ChdCs are enzymes involved in the prokaryotic heme biosynthesis pathway mainly of monoderm bacteria, but some diderm or intermediate representatives also use this pathway. They catalyze the hydrogen peroxide–driven oxidative decarboxylation of iron coproporphyrin III (coproheme) to iron protoporphyrin IX (heme b). After initial oxidation of coproheme to Compound I (two-electron deficient reaction intermediate), a catalytic tyrosine radical is generated, which is completely essential for both decarboxylation reactions. Mechanistic studies revealed the order of decarboxylation and proved that propionate at position 2 (p2) is decarboxylated first.

Exchange of Y135 with a tryptophan, in order to mirror the situation in the active site, led to a very inactive variant (data not shown), we therefore eliminated Y135 by inserting an alanine residue (Y135A), as has proven to keep the formation of Compound I perfectly intact in previous studies. The structures clearly show that the introduced amino acids occupy the positions of the respective residues in the wild-type protein. While the distance between Y135 and Cß-p2 is about 3.1 Å in the wild-type structure, the Y183 oxygen lies about 4.4 Å above the Cß of p4. Both single mutations leave the active site and the overall structure is unaffected. Y135A, in contrast, exhibits a very similar UV–Vis spectrum to the wild type (Soret maximum at 391 with a shoulder, visible bands at 490 and 631 nm) but shows no spectral shift of the Soret maximum upon titration with H2O2. Instead, an absorbance decrease of the Soret maximum and emergence of a single band at 580 nm are observed. As there is a lack of catalytic Y135, no decarboxylation activity with H2O2 is observed in this variant. Y135A is unable to perform the decarboxylation reaction on coproheme. This variant will form Compound I in the presence of H2O2 and, due to the lack of the catalytic tyrosine for Compound I* formation, the variant will instead oxidize coproheme to get back to the ferric resting state.

>[5x]GPMAEKLNFEELNSMQRYSQFAVFRAIPGALGSDRAEIVAQAQSFFDGLETAGKVEVRGIYDLAGCRAEADFMIWWIAEEFEEIQAAFARFRRETVLGQVSEVAWLGNSLHRPAEFNRSHLPSFIMGEIPGDWITVAPFVRSYDWYIMDPQKRRKILAEHGQAARDFPDVRANTVPAFALGDYEWMLAFEAPRLDRIVDLMHKMRYTEARLHVREETPFFTGRRVSEVSELVNVLPG>[4x]GSHMTEAEYLANYDPKAFKAQLLTVDAVLFTY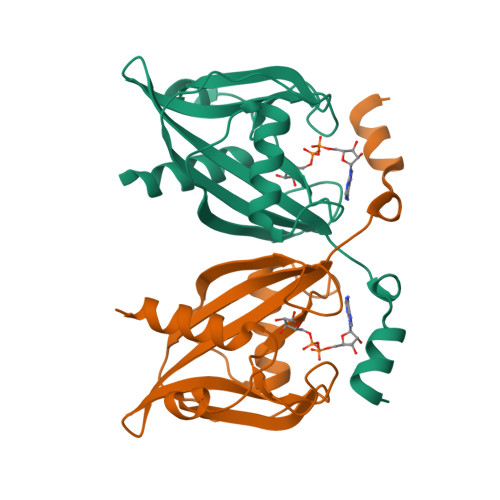HDQQLKVLLVQRSNHPFLGLWGLPGGFIDETCDESLEQTVLRKLAEKTAVVPPYIEQLCTVGNNSRDARGWSVTVCYTALMSYQACQIQIASVSDVKWWPLADVLQMPLAFDHLQLIEQARERLTQKALY> MEGDDLFDEFGNLIGVDPFDSDEEESVLDEQEQYQTNTFEGSGNNNEIESRQLTSLGSKKELGISLEHPYGKEVEVLMETKNTQSPQTPLVEPVTERTKLQEHTIFTQLKKNIPKTRYNRDYMLSMANIPERIINVGVIGPLHSGKTSLMDLLVIDSHKRIPDMSKNVELGWKPLRYLDNLKQEIDRGLSIKLNGSTLLCTDLESKSRMINFLDAPGHVNFMDETAVALAASDLVLIVIDVVEGVTFVVEQLIKQSIKNNVAMCFVINKLDRLILDLKLPPMDAYLKLNHIIANINSFTKGNVFSPIDNNIIFASTKLGFTFTIKEFVSYYYAHSIPSSKIDDFTTRLWGSVYYHKGNFRTKPFENVEKYPTFVEFILIPLYKIFSYALSMEKDKLKNLLRSNFRVNLSQEALQYDPQPFLKHVLQLIFRQQTGLVDAITRCYQPFELFDNKTAHLSIPGKSTPEGTLWAHVLKTVDYGGAEWSLVRIYSGLLKRGDTVRILDTSQSESRQKRQLHDISKTETSNEDEDSKTETPSCEVEEIGLLGGRYVYPVHEAHKGQIVLIKGISSAYIKSATLYSVKSKEDMKQLKFFKPLDYITEAVFKIVLQPLLPRELPKLLDALNKISKYYPGVIIKVEESGEHVILGNGELYMDCLLYDLRASYAKIEIKISDPLTVFSESCSNESFASIPVSNSISRLGEENLPGLSISVAAEPMDSKMIQDLSRNTLGKGQNCLDIDGIMDNPRKLSKILRTEYGWDSLASRNVWSFYNGNVLINDTLPDEISPELLSKYKEQIIQGFYWAVKEGPLAEEPIYGVQYKLLSISVPSDVNIDVMKSQIIPLMKKACYVGLLTAIPILLEPIYEVDITVHAPLLPIVEELMKKRRGSRIYKTIKVAGTPLLEVRGQVPVIESAGFETDLRLSTNGLGMCQLYFWHKIWRKVPGDVLDKDAFIPKLKPAPINSLSRDFVMKTRRRKGISTGGFMSNDGPTLEKYISAE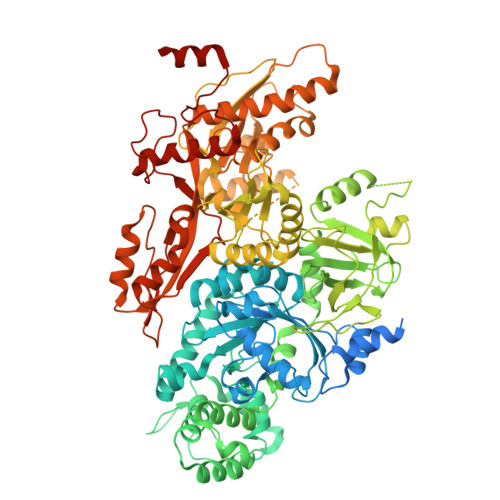LYAQLRENGLVP> AGFCCPSHWSSYDRYCYKVFKQEMTWADAEKFCTQQHTGSHLVSFHSTEEVD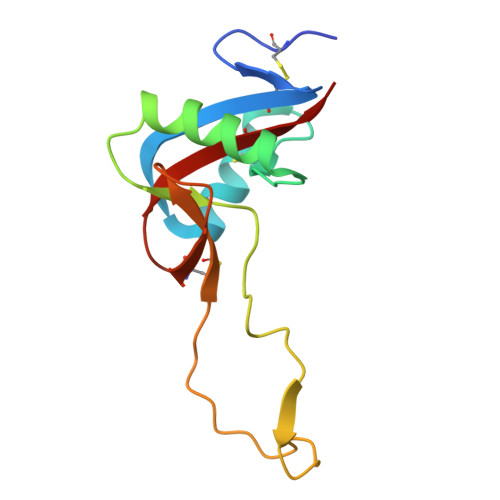FVVKMTHQSLKSTFFWIGANNIWNKCNWQWSDGTKPEYKEWHEEFECLISRTFDNQWLSAPCSDTYSFVCKFEA oligomycin C | 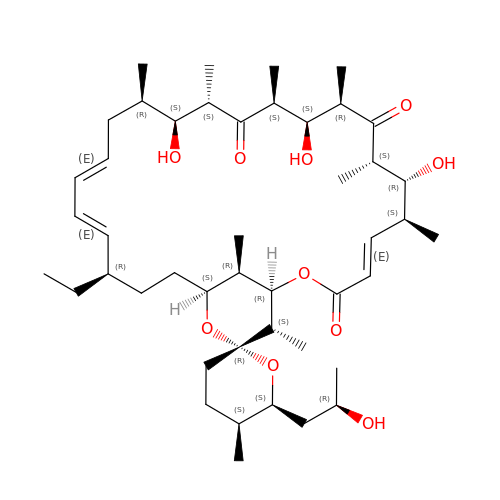C45 H74 O10 | CMMLZMMKTYEOKV-RDKHTNMBSA-N> AMGKCPTKVVLLRNMVGAGEVDEDLEVETKEECEKYGKVGKCVIFEIPGAPDDEAVRIFLEFERVESAIKAVVDLNGRYFGG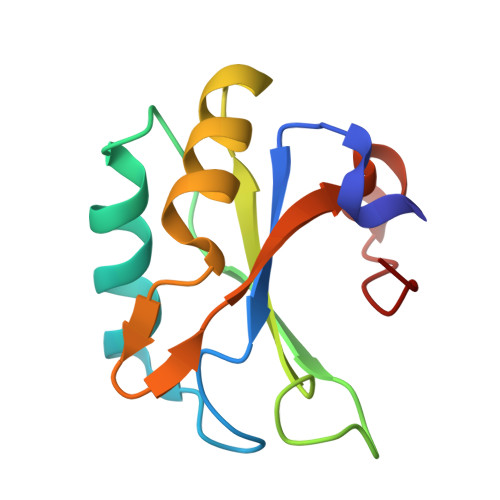RVVKACFYNLDKFRVLDLAEQV> MVTSNVVLVSGEGERFTVDKKIAERSLLLKNYLNDASGDDDDEDDDEIVMPVPNVRSSV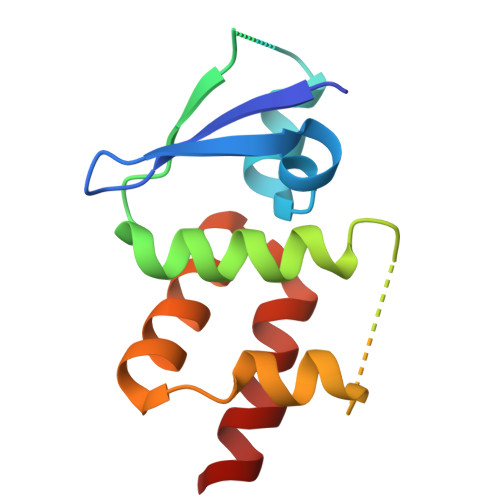LQKVIEWAEHHRDSNFPDEDDDDSRKSAPVDSWDREFLKVDQEMLYEIILAANYLNIKPLLDAGCKVVAEMI>[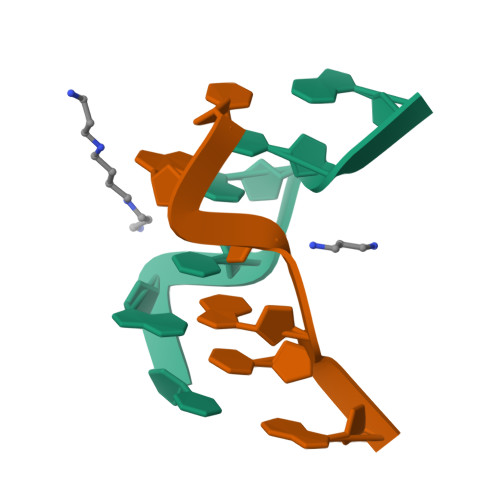2x]CACGTG>[2x]GSHMDKSFSNYFWGANDEGYHALLSR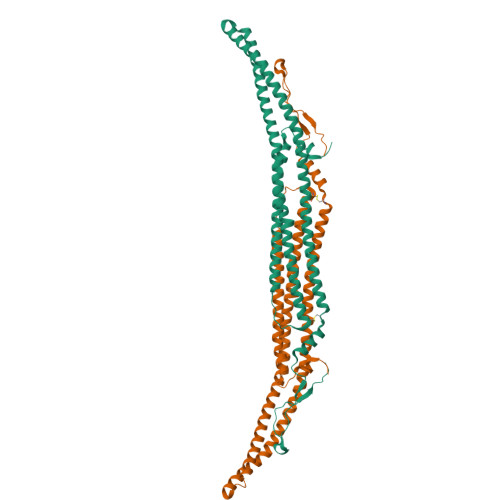FSDVKHINEELRSFYHERANIEEDYAKRMAKLSRTTFSSLETGCLKESVQVMKAEVDNMAKSHLQISQLLQDDVENAFTRYAASLKDKKKMIVSGIEKVHKDKLSKHQALVKAQDKYHYLCKKVNYYVSQQNMLFGKELEKNNAKLNKTQNAITASSSDYQSAVAAVRDSYARWTNEWRSTCDKLQDIEEERRHFLKSVMWTFTLLISRSCFNDDQACERIRKNLEQCSVSQDVLEFIDAKSTGTGIPQPPKFYDYYKGEVPDDSVELVQANFQRAQTKIENDN>[2x]MIVLFVDFDYFYAQVEEVLNPSLKGKPVVVCVFSGRFEDSGAVATANYEARKFGVKAGIPIVEAKKILPNAVYLPMRKEVYQQVSSRIMNLLREYSEKIEIASIDEA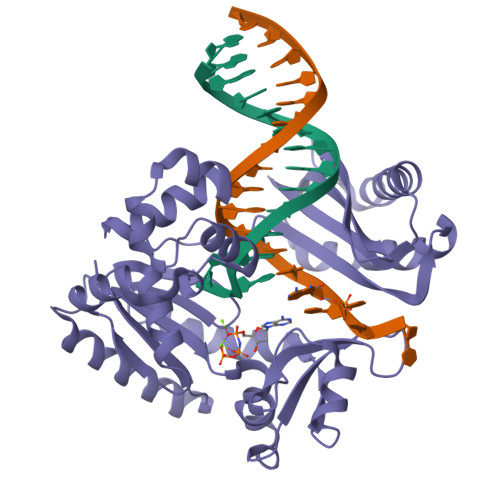YLDISDKVRDYREAYNLGLEIKNKILEKEKITVTVGISKNKVFAKIAADMAKPNGIKVIDDEEVKRLIRELDIADVPGIGNITAEKLKKLGINKLVDTLSIEFDKLKGMIGEAKAKYLISLARDEYNEPIRTRVRKSIGRIVTMKRNSRNLEEIKPYLFRAIEESYYKLDKRIPKAIHVVAVTEDLDIVSRGRTFPHGISKETAYSESVKLLQKILEEDERKIRRIGVRFSKFI> MATRGIRNNNPGNIRVSKDQWEGMTGDDGAFVTFDSPESGVRALGKNLLSYGRQGYDSIEKIINRWA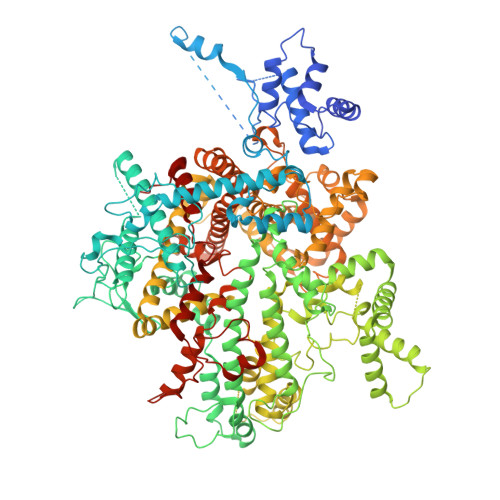PPNENDTKAYIDSVVAATGIPATQSLDLSNQDTLSALAQAISFHETGSRYDPEVYQKGVARALNGISPKTPPVSANVFDALTEGLKAKPKVALGENLPTAAGLNIEGQAPEAPNESFGEMFYKSTGETMQEREDRSTWFGFGAATEAEVKNSMVGVAIRAGQTEDSLDVIGDVFNPTRWNNHKWTREELDQIRNAGVLPQYYGVITGGSPQNLTELINLALENQKLDQEKAKAGTGAQLAAGVIGAGVDPLTYVPIAGQVGKGGKLVNKMFTVAAQSGALAGVSEMARTSVAGGDAHVAEAILGGALFGGGMTAIADGLGRALGRNTNEFAGPATRLEARETARNVDGQDLSRLPIQEGEQTFSHQGVKFADVPNEPGSVRLEDGSILIGENPLNPKTRQVFDEVIEPERAAAGVNLGGLTEIGLKLLRSENPEIRGVAADLVRSPTGMQSGASGKIGTTASDVFERLRAVDHRFYNDIDDAVTEALKDPYFQTAFWRDSGAFRQDIYQRVSMAIEDGSGNLKAELTPGELKVYDLLKNQFDAKREMMENPAMFGRPDAQSIFPGSRFKGTYVPHVYSSQMKELYIKELGSPEALQEAIKKSWLTSYASRPEVKKRVDEALLEADPTLTPEGLAAAVDKYANDKAYGISHTEQFERSSVMEENINGLVGLENNSFLEARNLFDSDMSIVLPNGQTFSVNNLREWDMDKIVPAYNRRVNGDIAIMAGTGKTTKEMKDLVETLMNKAGDDGKLKGEVSTLRDTLKILTGRARRDGADDAAFATVMRTMTDLAFFAKNAYMGVQNLTEIGGMLARGNVRAMLHGVPMFRDLAFRNKKVGASEIKDLHNVIFGKELDDSIRPSKQDVIDRLRSYSDLGRGAATALGTAKYYTGELAVRSPFTKVLNGTTNYLLDAGRQGFLSDIVEHSLTGSKRRFDDRWLKTAGISDEQWKGIKSLIRESVTRGPDGKYTIKDKKAFSQDQRAMDLWRMGDTIADETLLRPHKLSNMDAKAYGPIAKTVLQFKNFVIKSINGRTMRTFYNATKNNRAMDAALSTVMSMGLAGMYYMAQAHIKAYAMQDGRDREYLKQALNPTMIGYAALSRSSHLGGPLGVANILGGIAGYEDTKMLRSSILPRSPTEKTEKPIAFGAASSGPVMNVVGNFLEQVPAFGYAANVGATAYNLAGYLKADTRVNERDYMTGMYNTFRELVPNDPITQKLLLGTFEEQGIHIKD>GAV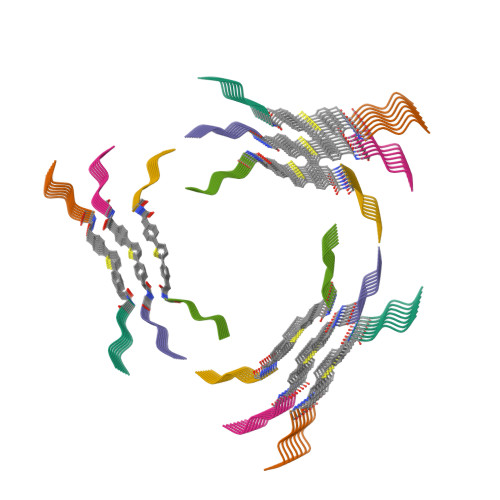EV[6x]> MSREEVESLIQEVLEVYPEKARKDRNKHLAVNDPAVTQSKKCIISNKKSQPGLMTIRGCAYAGSKGVVWGPIKDMIHISHGPVGCGQYS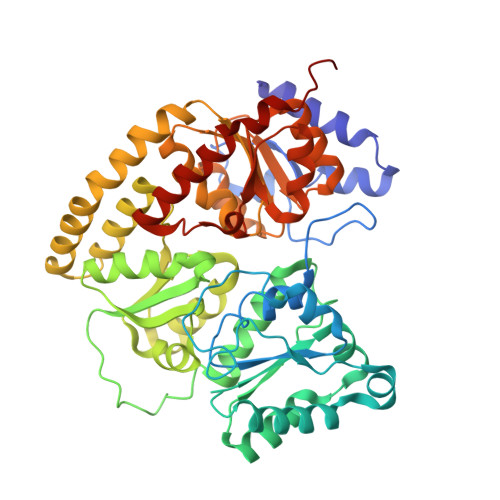RAGRRNYYIGTTGVNAFVTMNFTSDFQEKDIVFGGDKKLAKLIDEVETLFPLNKGISVQSECPIGLIGDDIESVSKVKGAELSKTIVPVRCEGFRGVSQSLGHHIANDAVRDWVLGKRDEDTTFASTPYDVAIIGDYNIGGDAWSSRILLEEMGLRCVAQWSGDGSISEIELTPKVKLNLVHCYRSMNYISRHMEEKYGIPWMEYNFFGPTKTIESLRAIAAKFDESIQKKCEEVIAKYKPEWEAVVAKYRPRLEGKRVMLYIGGLRPRHVIGAYEDLGMEVVGTGYEFAHNDDYDRTMKEMGDSTLLYDDVTGYEFEEFVKRIKPDLIGSGIKEKFIFQKMGIPFRQMHSWDYSGPYHGFDGFAIFARDMDMTLNNPCWKKLQAPWE(2R)-5-[(carbamoyloxy)methyl]-2-[(1R)-1-{[(2Z)-2-(furan-2-yl)-2-(methoxyimino)acetyl]amino}-2-oxoethyl]-3,6-dihydro-2H-1,3-thiazine-4-carboxylic acid | C16 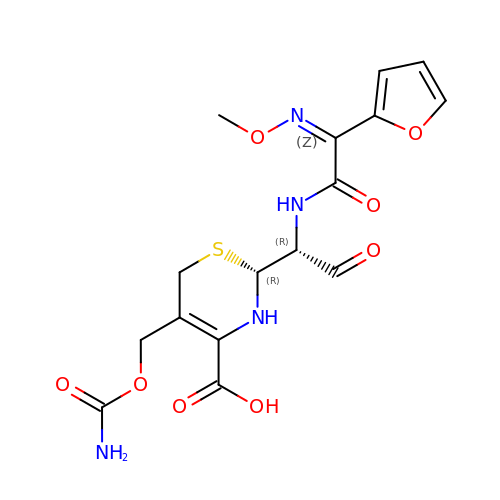H18 N4 O8 S | RUUDYXYLGTZCPN-VRVPSKPHSA-N>MNDLERLFNPSAIAVVGASKDPSKIGSQILRNLLSYGFKGKVYPINPTADELMGLKCYPKVSDVPDKVDVAVISVPSDKVLGVIDDCGKAGVKFAVVITSGFKEVGNEELEEELVRRAHSYGMRVLGPNIFGYLYAPARLNATFGPKDVLSGNVAFISQSGALGIALMGYTVVENIGISSIVSVGNKADLDDVDLLDFFDKDPNTGVIMIYLEGIAPGRGRMFIDVASRVSLRKPIIVIKAGRTEVGARAAASHTGSIAGSVAIYESAFKQSGILMAKSVEDAFDWTKALSWNPIPEGERLIVLTNGGGAGVQSTDTFADNGIYLSKPPESLIQEIKKFVPPFASFANPIDITGMAPDDWYYMGTLAALKNPDVDALTV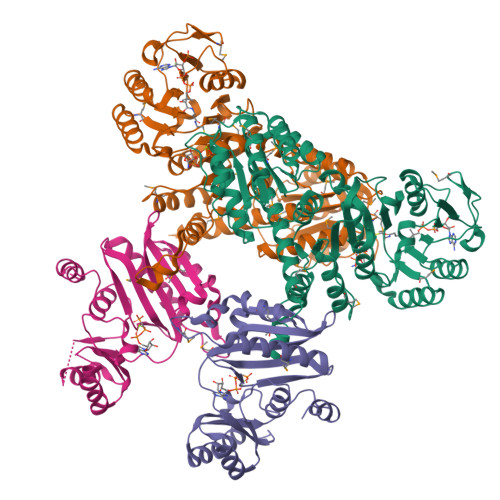LYCQTAVTTPIGVAKGIVDAIKEAGNSKPVTVGMVGGPEVAEAVSFLNKQRIAAYPTPERASSAMSALYAYARARSYVMKSLAVR[2x];>[2x]MSSRDLLLKAKENGRKSLLEHEAKYFISSYGIPVTNIRLAKSEEEAVNFSREIGFPVVLKIVSPQVVHKSDVGGVKVNLRSEEEVRKAYREIIENVKRNVPNAEIEGILVQEFAPPGVELIIGLLRDPQFGPTVMFGLGGVFVELFRDVSFRVAPLSEQDAESMIKEVKAYKLLTGFRGMEPVDIEAIKDALIRAGRIGVENEEIAEMDLNPVIAYPKGIKVVDARIILR> MRGKIYDRNGKVLAEDVERYKLVAVIDKKASANSKKPRHVVDKKETAKKLSTVINMKPEEIEKRLSQKKAFQIEFGRKGTNLTYQDKLKIEKMNLPGISLLPETERFYPNGNFASHLIGRAQKNPDTGELKGALGVEKIFDSYLSGSKGSLRYIHDIWGYIAPNTKKEKQPKRGDDVHLTIDSNIQVFVEEALDGMVERYQPKDLFAVVMDAKTGEILAYSQRPTFNPETGKDFGKKWANDLYQNTYEPGSTFKSYGLAAAIQEGAFDPDKKYKSGHRDIMGSRISDWNRVGWGEIPMSLGFTYSSNTLMMHLQDLVGADKMKSWYERFGFGKSTKGMFDGEAPGQIGWSNELQQKTSSFGQSTTVTPVQMLQAQSAFFNDGNMLKPWFVNSVENPVSKRQFYKGQKQIAGKPITKDTAE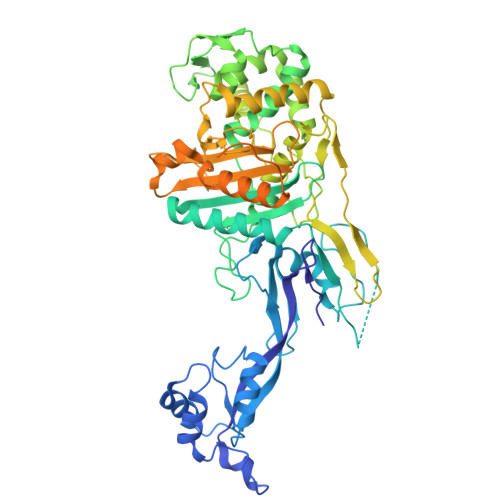KVEKQLDLVVNSKKSHAANYRIDGYEVEGKTGTAQVAAPNGGGYVKGPNPYFVSFMGDAPKKNPKVIVYAGMSLAQKNDQEAYELGVSKAFKPIMENTLKYLNVGKSKDDTSNAEYSKVPDVEGQDKQKAIDNVSAKSLEPVTIGSGTQIKAQSIKAGNKVLPHSKVLLLTDGDLTMPDMSGWTKEDVIAFENLTNIKVNLKGSGFVSHQSISKGQKLTEKDKIDVEFSS>AVVQRVEIHKLRQGENLILGFSIGGGIDQDPSQNPFSEDKTDKGIYVTRVSEGGPAEIAGLQIGDKIMQVNGWDMTMVTHDQARKR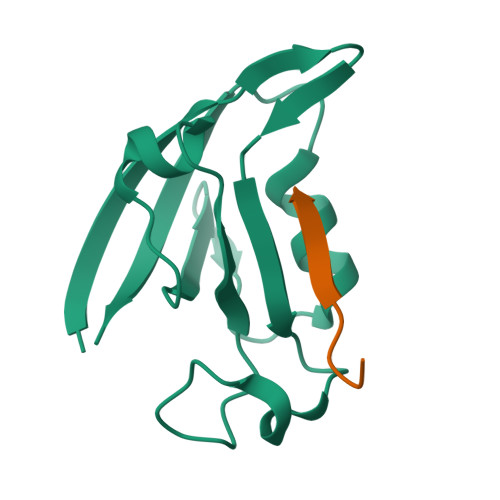LTKRSEEVVRLLVTRQ[2x];>ANSRWPTSIL[2x]> SNASIVSLLGIKVLNNPAKFTDPYEFEITFECLESLKHDLEWKLTYV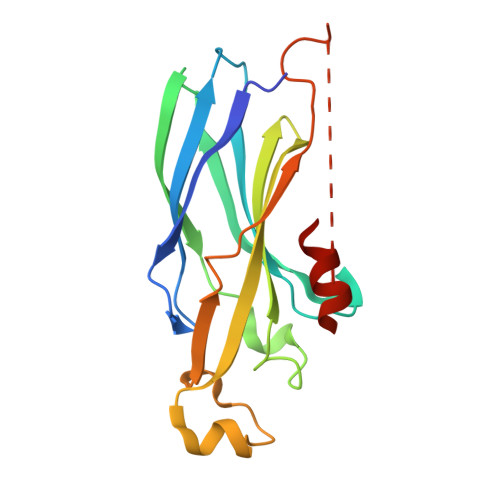GSSRSLDHDQELDSILVGPVPVGVNKFVFSADPPSAELIPASELVSVTVILLSCSYDGREFVRVGYYVNNEYDEEELRENPPAKVQVDHIVRNILAEKPRVTRFNIVWDNAAGAATAAKKEIKLARRLRGER>[2x]MTSITPVTLANCEDEPIHVPGAIQP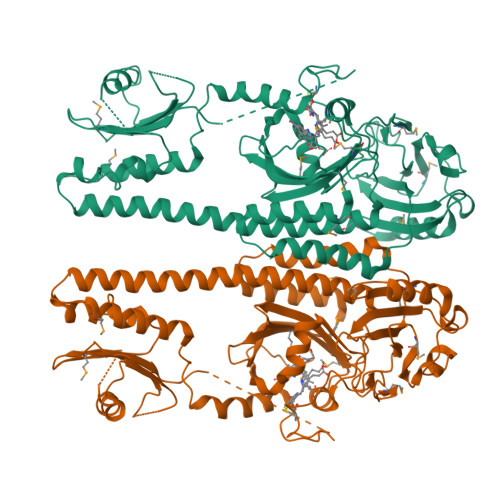HGALVTLRADGMVLAASENIQALLGFVASPGSYLTQEQVGPEVLRMLEEGLTGNGPWSNSVETRIGEHLFDVIGHSYKEVFYLEFEIRTADTLSITSFTLNAQRIIAQVQLHNDTASLLSNVTDELRRMTGYDRVMAYRFRHDDSGEVVAESRREDLESYLGLRYPASDIPAQARRLYIQNPIRLIADVAYTPMRVFPALNPETNESFDLSYSVLRSVSPIHCEYLTNMGVRASMSISIVVGGKLWGLFSCHHMSPKLIPYPVRMSFQIFSQVCSAIVERLEQGRIAELLRVSTERRLALARRARDADDLFGALAHPDDGIAALIPCDGALVMLGGRTLSIRGDFERQAGNVLQRLQRDPERDIYHTDNWPQPSEDSPDGGDCCGVLAIRFHRQESGWIFWFRHEEVHRIRWGGKPEKLLTIGPSGPRLTPRGSFEAWEEVVRGHSTPWSETDLAIAEKLRLDLMELCLNHALEHHHHHH Phosphoribosyl pyrophosphate synthetase (PRPS) stands as the first and rate-limiting enzyme in the purine biosynthesis pathway. It catalyzes the pyrophosphorylation of D-ribose-5-phosphate (R5P), obtained from the glucose pentose phosphate pathway (PPP), at the 1’ hydroxyl group position, yielding the catalytic product 5-phosphoribosyl-ɑ-1-pyrophosphate (PRPP). PRPP serves as an essential metabolic intermediate for purine biosynthesis via both de novo and salvage pathways, as well as for the synthesis of pyrimidines, amino acids (tryptophan and histidine), and co-factors (NAD+ and NADP+). Conversely, PRPS2 displays ~94% identity with PRPS1 and shares exactly the same biochemical reaction.

In addition to conventional enzymatic catalysis, PRPS enzymes are downregulated through allosteric feedback inhibition by downstream nucleotide biosynthesis products ADP or GDP21. To avoid potential confusing, we chose to use GDP instead to ADP specifically for the allosteric inhibition regulation study as GDP does not bind to the catalytic pocket as a substrate competitor. To explain these unexpected variations, we determined the structure of PRPS1 in complex with R5P, ApCpp, Cd2+ ion, and GDP by co-crystallization. The GDP ligand was positioned at the allosteric site between Loop2 and the C-terminal α12’ helix of PRPS1 with pocket volume 33 Å3, stabilizing the conformations of Loop2 and the α12’ helix for catalysis. Strikingly, in vitro feedback inhibition assays indicated that the enzymatic activity of PRPS1 was inhibited by GDP with an IC50 value of 706 µM, while that of PRPS2 was unaffected by up to 10 mM GDP, suggesting that PRPS2 was insensitive to feedback inhibition. Indeed, PRPS2 binds with GDP with extremely weak affinity (Kd > 200 µM), whereas PRPS1 bound GDP with a Kd value of 10 µM. In contrast, 3AA in PRPS2 sterically blocked GDP binding at the allosteric site, abolishing the feedback inhibition response of PRPS2.

>[6x]SPNIKIFSGSSHQDLSQKIADRLGLELGKVVTKKFSNQETCVEIGESVRGEDVYIVQSGCGEINDNLMELLIMINACKIASASRVTAVIPCFPYARQDKKDKSRAPISAKLVANMLSVAGADHIITMDLHASQIQGFFDIPVDNLYAEPAVLKWIRENISEWRNCTIVSPDAGGAKRVTSIADRLNVDFALIHKERKKANEVDRMVLVGDVKDRVAILVDDMADTCGTICHAADKLLSAGATRVYAILTHGIFSGPAISRINNACFEAVVVTNTIPQEDKMKHCSKIQVIDISMILAEAIRRTHNGESVSYLFSHVPL5-CHLORO-4-OXOPENTANOIC ACID | C5 H7 Cl 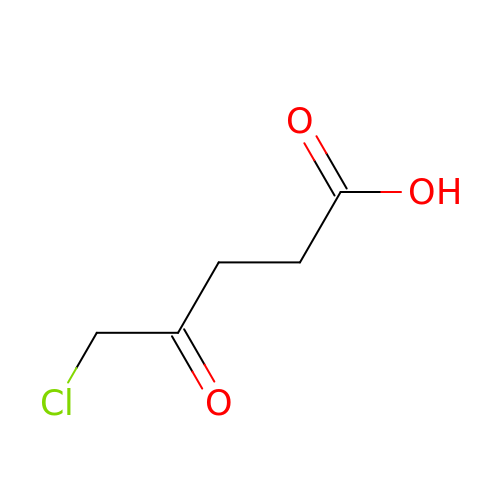O3 | NDODXPYZKSROJQ-UHFFFAOYSA-N>[4x]MVDKHEEITLPIVLSCNYQSDITYPGQKQFDCGNPVIDKFVRASLKKSVRNSDCAAKALIDRQSGELIGICTFTAYSLEKQRVSGVLQGSQPSEIG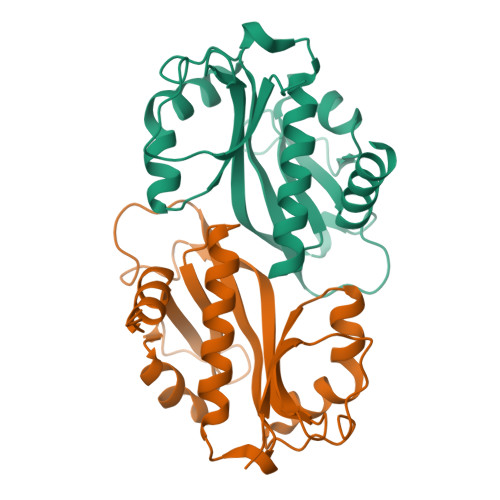VVRLVMLGVARKYQKRGFDQDLLCDFFEHVKIIHQALPIKGVYLDADPAAINFYARLGFVQLSATPNAFGAVPMFLAIQHILAALEHHHHHH> SD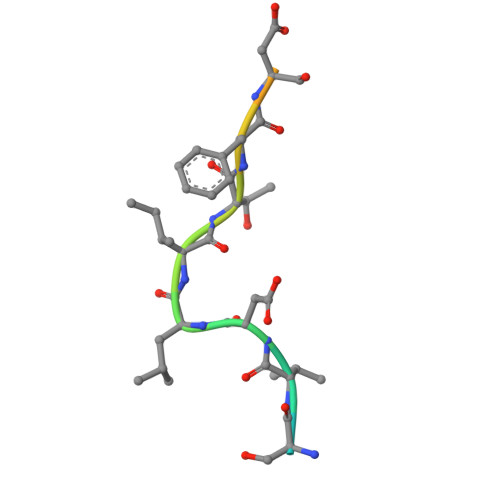HSVDLITFDSVTDIY> GAMGDVSRLNQRNINELKIFVEKAKYYSIKLDAIYNECTGAYNDIMTYSEGTFSDQSKVNQAISIFKKDNKIVNKFKELEKIIEEYKPMFLSKLIDDFAIELDQAVDNDVSNARHVADSYKKLRKSVVLAYIESFDVISSKFVDSKFVEASKKFVNKAKEFVEENDLIALESIVKTIGDMVNDREINSRSRANNFAKKEADFLGAAVELEGAYKAIKQTLL

Lyme borreliae produce other outer surface proteins, including CspZ (also known as BbCRASP-228,29). CspZ promotes bacterial dissemination to distal tissues by evading the complement system, the first-line innate immune defense in vertebrates in the blood, through binding and recruiting a host complement inhibitor, factor H (FH). Additionally, CspZ is only produced after Lyme borreliae invade vertebrate hosts and, as such, induces CspZ-specific immune responses after natural infection. Similar to CspZ, CspZ-YA is an all-α-helical protein composed of nine α-helices (denoted as helices A to I).

Additionally, to avoid the formation of intermolecular disulfide bonds, resulting in the risk of protein aggregations, we substituted two cysteine residues, C53S and C187S, to generate untagged CspZ-YAC53S and CspZ-YAC187S. We also determined the crystal structure of CspZ-YAC187S at 1.95 Å resolution. Superimposed structures of CspZ-YA, CspZ-YAC187S, and CspZ-YAI183Y, using CCP4MG software, showed no significant differences in surface epitopes. We found a water molecule present in the space between helix I and C187 of CspZ-YA, as well as between helix I and S187 of CspZ-YAC187S. That water molecule does not impact the intramolecular interactions in CspZ-YA, but coordinates the interactions with S187 on the helix H and E214 on the helix I via hydrogen bonding in CspZ-YAC187S(dotted lines in Fig. 6B), likely enhancing the protein stability. Thus, the highly polar nature of serine together with a slightly smaller footprint of oxygen from S187 may be the cause of the water molecule positioning in the fashion to enhance hydrogen bond-mediated intramolecular interactions in CspZ-YAC187S. Thus, the results here identified a less flexible loop region between helices H and I (R5; residues 198–221) in the CspZ-YAC187S and CspZ-YAI183Y, compared to CspZ-YA. In contrast, the Tm-values of CspZ-YA were significantly lower, 57.5 and 58.4 °C for histidine-tagged and untagged CspZ-YA, respectively, indicating a stability enhancement through mutagenesis. However, CspZ-YA but not CspZ-YAI183Y and CspZ-YAC187S previously incubated at 37 °C for 24-h had 1.6-fold lower levels of recognition, compared to those proteins prior to incubation, even though SEC-HPLC did not indicate significant aggregation or degradation (results not shown).>MSLDTIKVGILGYGLSGSVFHGPLLDVLDEYQISKIMTSRTEEVKRDFPDAEVVHELEEITNDPAIELVIVTTPSGLHYEHTMACIQAGKHVVMEKPMTATAEEGETLKRAADEKGVLLSVYHNRRWDNDFLTIKKLISEGSLEDINTYQVSYNRYRPEVQARWREKEGTATGTLYDLGSHIIDQTLHLFGMPKAVTANVMAQRENAETVDYFHLTLDYGKLQAILYGGSIVPANGPRYQIHGKDSSFIKYGIDGQEDALRAGRKPEDDSWGADVPEFYGKLTTIRGSDKKTETIPSVNGSYLTYYRKIAESIREGAALPVTAEEGINVIRIIEAAMESSKE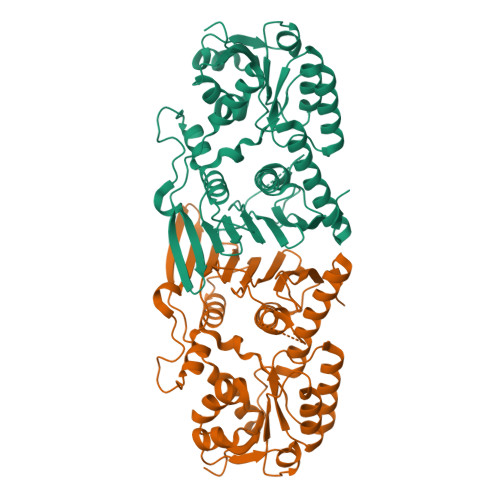KRTIMLEHEGHHHHHH[2x]>[2x]GHMDITEERLHYQVGQRALIQAMQISAMPELVEAVQKRDLARIKALIDPMRSFSDATYITVGDASGQRLYHVNPDEIGKSMEGGDSDEALIN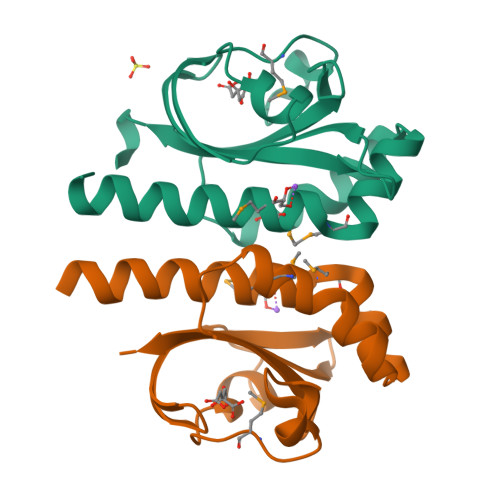AKSYVSVRKGSLGSSLRGKSPIQDATGKVIGIVSVGYTIEQLE αHBs are oligomers of 5 or more α-helical peptides that assemble into coiled-coil structures with central solvent-accessible channels. We targeted two properties of αHBs: oligomeric state, which directly affects the internal diameter of the channel; and the identities of channel-facing residues, which fine tune this dimension and introduce different chemistries. The αHBs are loaded with an environment sensitive dye (in this case, 1,6-diphenyl-1,3,5-hexatriene, DPH) that binds within the channels and fluoresces. Accordingly, challenging the array with analytes leads to differential displacement of the dye across the array to give a fluorescent fingerprint.

Despite the requirements for aliphatic residues at a and d, up to 40% of these can be changed to other side chains without compromising barrel integrity. We introduced mutations at one or two of these sites to generate four groups of αHB: Group I had entirely hydrophobic interiors, but with different sizes and shapes of channel; Groups II and III had polar uncharged or polar charged residues, respectively, at specific points along the channel; and Group IV had aromatic residues installed in their channels. In detail, the sixteen Group I peptides included: previous designs for a pentamer, 3 hexamers, 2 heptamers and an octamer all verified by X-ray crystallography;27,29 single and/or double mutations to Ala and Gly at central a and d sites to generate larger channels; a single-Pro mutant at the final d site to kink and open the C-terminal end of the channel; and a variant with all a sites made Met to vary the hydrophobic chemistry used. Finally, one third of the designs were crystallized and yielded 12 X-ray crystal structures, all of which were open αHBs with fully accessible channels. Conversely, the FAs generate signal through interactions with the more-hydrophobic and aromatic-containing channels (Group I and IV).

>[7x]XGEIAQAMKEIAKAMKEIAWAMKEIAQAMKGX>MALVLEIFTLLASICWVSANIFEYQVDAQPLRPCELQRETAFLKQADYVPQCAEDGSFQTVQCQNDGRSCWCVGANGSEVLGSRQPGRPVACLSFCQLQKQQILLSGYINSTDTSYLPQCQDSGDYAPVQCDVQQVQCWCVDAEGMEVYGTRQLGRPKRCPRSCEIRNRRLLHGVGDKSPPQCSAEGEFMPVQCKFVNTTDMMIFDLVHSYNRFPDAFVTFSSFQRRFPEVSGYCHCADSQGRELAETGLELLLDEIYDTIFAGLDLPSTFTETTLYRILQRRFLAVQSVISGRFRCPTKCEVERFTATSFGHPYVPSCRRNGDYQAVQCQTEGPCWCVDAQGKEMHGTRQQGEPPSCAEGQSCASERQQALSRLYFGTSGYFSQHDLFSSPEKRWASPRVARFATSCPPTIKELFVDSGLLRPMVEGQSQQFSVSENLLKEAIRAIFPSRGLARLALQFTTNPKRLQQNLFGGKFLVNVGQFNLSGALGTRGTFNFSQFFQQLGLASFLNGGRQEDLAKPLSVGLDSNSSTGTPEAAKKDGTMNKPTVGSFGFEINLQENQNALKFLASLLELPEFLLFLQHAISVPEDVARDLGDVMETVLSSQTCEQTPERLFVPSCTTEGSYEDVQCFSGECWCVNSWGKELPGSRVRGGQPRCPTDCEKQRARMQSLMGSQPAGSTLFVPACTSEGHFLPVQCFNSECYCVDAEGQAIPGTRSAIGKPKKCPTPCQLQSEQAFLRTVQALLSNSSMLPTLSDTYIPQCSTDGQWRQVQCNGPPEQVFELYQRWEAQNKGQDLTPAKLLVKIMSYREAASGNFSLFIQSLYEAGQQDVFPVLSQYPSLQDVPLAALEGKRPQPRENILLEPYLFWQILNGQLSQYPGSYSDFSTPLAHFDLRNCWCVDEAGQELEGMRSEPSKLPTCPGSCEEAKLRVLQFIRETEEIVSASNSSRFPLGESFLVAKGIRLRNEDLGLPPLFPPREAFAEQFLRGSDYAIRLAAQSTLSFYQRRRFSPDDSAGASALLRSGPYMPQCDAFGSWEPVQCHAGTGHCWCVDEKGGFIPGSLTARSLQIPQCPTTCEKSRTSGLLSSWKQARSQENPSPKDLFVPACLETGEYARLQASGAGTWCVDPASGEELRPGSSSSAQCPSLCNVLKSGVLSRRVSPGYVPACRAEDGGFSPVQCDQAQGSCWCVMDSGEEVPGTRVTGGQPACESPRCPLPFNASEVVGGTILCETISGPTGSAMQQCQLLCRQGSWSVFPPGPLICSLESGRWESQLPQPRACQRPQLWQTIQTQGHFQLQLPPGKMCSADYADLLQTFQVFILDELTARGFCQIQVKTFGTLVSIPVCNNSSVQVGCLTRERLGVNVTWKSRLEDIPVASLPDLHDIERALVGKDLLGRFTDLIQSGSFQLHLDSKTFPAETIRFLQGDHFGTSPRTWFGCSEGFYQVLTSEASQDGLGCVKCPEGSYSQDEECIPCPVGFYQEQAGSLACVPCPVGRTTISAGAFSQTHCVTDCQRNEAGLQCDQNGQYRASQKDRGSGKAFCVDGEGRRLPWWETEAPLEDSQCLMMQKFEKVPESKVIFDANAPVAVRSKVPDSEFPVMQCLTDCTEDEACSFFTVSTTEPEISCDFYAWTSDNVACMTSDQKRDALGNSKATSFGSLRCQVKVRSHGQDSPAVYLKKGQGSTTTLQKRFEPTGFQNMLSGLYNPIVFSASGANLTDAHLFCLLACDRDLCCDGFVLTQVQGGAIICGLLSSPSVLLCNVKDWMDPSEAWANATCPGVTYDQESHQVILRLGDQEFIKSLTPLEGTQDTFTNFQQVYLWKDSDMGSRPESMGCRKDTVPRPASPTEAGLTTELFSPVDLNQVIVNGNQSLSSQKHWLFKHLFSAQQANLWCLSRCVQEHSFCQLAEITESASLYFTCTLYPEAQVCDDIMESNAQGCRLILPQMPKALFRKKVILEDKVKNFYTRLPFQKLMGISIRNKVPMSEKSISNGFFECERRCDADPCCTGFGFLNVSQLKGGEVTCLTLNSLGIQMCSEENGGAWRILDCGSPDIEVHTYPFGWYQKPIAQNNAPSFCPLVVLPSLTEKVSLDSWQSLALSSVVVDPSIRHFDVAHVSTAATSNFSAVRDLCLSECSQHEACLITTLQTQPGAVRCMFYADTQSCTHSLQGQNCRLLLREEATHIYRKPGISLLSYEASVPSVPISTHGRLLGRSQAIQVGTSWKQVDQFLGVPYAAPPLAERRFQAPEPLNWTGSWDASKPRASCWQPGTRTSTSPGVSEDCLYLNVFIPQNVAPNASVLVFFHNTMDREESEGWPAIDGSFLAAVGNLIVVTASYRVGVFGFLSSGSGEVSGNWGLLDQVAALTWVQTHIRGFGGDPRRVSLAADRGGADVASIHLLTARATNSQLFRRAVLMGGSALSPAAVISHERAQQQAIALAKEVSCPMSSSQEVVSCLRQKPANVLNDAQTKLLAVSGPFHYWGPVIDGHFLREPPARALKRSLWVEVDLLIGSSQDDGLINRAKAVKQFEESRGRTSSKTAFYQALQNSLGGEDSDARVEAAATWYYSLEHSTDDYASFSRALENATRDYFIICPIIDMASAWAKRARGNVFMYHAPENYGHGSLELLADVQFALGLPFYPAYEGQFSLEEKSLSLKIMQYFSHFIRSGNPNYPYEFSRKVPTFATPWPDFVPRAGGENYKEFSELLPNRQGLKKADCSFWSKYISSLKTSADGAKGGQSAESEEEELTAGSGLREDLLSLQEPGSKTYSK[2x]

The thyroglobulin (TG) protein is essential to thyroid hormone synthesis, plays a vital role in the regulation of metabolism, development and growth and serves as intraglandular iodine storage. Thyroglobulin (TG) is a 660 kDa hyperglycosylated protein expressed in thyrocytes and secreted to the follicular lumen where it accumulates. TG is simultaneously a precursor for thyroid hormone (TH) biogenesis, the synthesis of which is itself modulated by thyroid-stimulating hormone (TSH) signaling, and the carrier protein responsible for iodine storage in the follicle colloid. Each chain is formed by regions I, II, and III and a C-terminal ChEL domain.

Here, we present the cryo-electron microscopy structure of native and fully glycosylated hTG from healthy thyroid glands to 3.2 Å resolution. A cryo-EM map at 3.2 Å nominal resolution was reconstructed allowing atomic modeling of the hTG dimer to around 90% completeness (2,483 modeled residues over 2,748 expected residues per chain). Poorly resolved parts of the map, in particular at the N-terminal and other flexible parts, prevented modeling of the full-length protein. This composite map is the result of a globally refined consensus map and two maps locally refined around particularly flexible regions, the “wing” (3.8 Å resolution) and the “foot” (4.1 Å resolution). The hTG dimer is ~250 Å long by 160 Å wide and 110 Å along the C2 symmetry axis. The interface between monomers buries an area of 31,100 Å2 involving all regions except region II. We identified 57 DSBs over the overall hTG structure stabilizing the protein and three types of cysteine-rich internal homology repeats in hTG: type 1, type 2 and type 3. The ChEL domains and repeats 1.6–1.8 form the core of the dimer and lie near the C2 symmetry axis while regions 2 and 3, as well as the remaining type 1 repeats, occupy more peripheral zones. We modeled 2 of the expected 4 hormonogenic sites, namely site B and site D. Acceptor tyrosines of sites A and C are located at the extreme N- and C-termini of the hTG chain and could not be modeled likely due to the inherent flexibility of these regions. Out of those, 14 asparagine residues showed an additional density in the map and N-linked glycan structures were modeled. Our structural characterization also evidences features of hTG that were previously unknown: the environment and possible function of the 4 NHIs present in type 1 repeats; the previously annotated linker region which in fact is a NHI of repeat 1.5; the globular nature of type 3 repeats, which could be annotated differently, and finally the flexible nature of the wing and foot regions.>MQNGDFQILDYTGLISTMPRVDTLLQSMNLFTEHFGRTTVARIERLDDGAGDIKAVQRGGVRQHLANDRKKIVNLNIPFFPLDRSIDRADIQNFREFGTENAPATVDAEVQRHMARIRRSHAILKSKAMYAALKGTSWSPDDPVSDYNYYDVWGATQTTADVDFTKLGVDPIEVLEAEARAHIIDWAGDNGDNYEIVVLASRQWFSALIAHPQVTGAYSQYPSTQEILRRRLGGNANNRIFEHKNILFIEDISGNIPAGEAYIFPRGISRMFEIYYAPSDTLRDANQAAQEL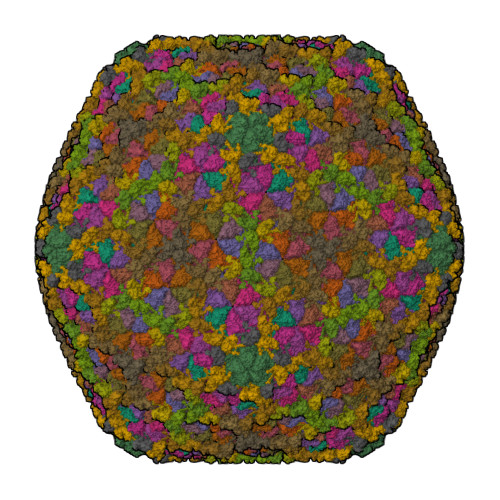YVFFKESNYLREAKIESETSFLTVNNRPELVVKSTGKFTA[13x];>MAKAHVATLEGNYSDIVLGRVVAFGDTGWNFKEVDMTFIADDADADSKTTLFAGVLVGEDGTPATAAAGVFGVLVDRKVLPGVDHYIGVFEPGEKVPMVLAVRGLTLNQLKLKYADGTAIDAAGIQALEAQGNQVTDKIVGTQFIGSVL[13x]> GSESDSGMASQADQKEEELLLFWTYIQAMLTNLESLSLDRIYNMLRMFVVTGPALAEIDLQELQGYLQKKVRDQ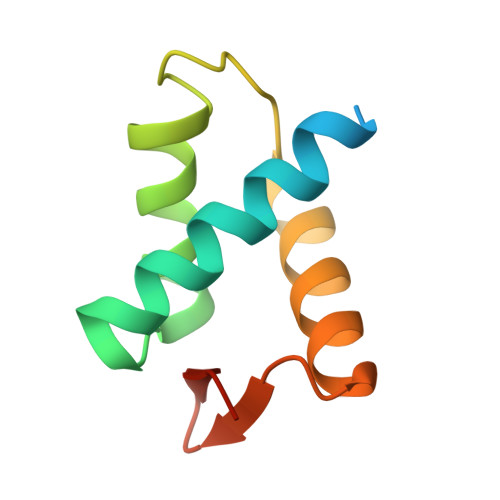QLVYSAGVYRLPKNCS> AMADLEQKVLEMEASTYDGVFIWKISDFPRKRQEAVAGRIPAIFSPAFYTSRYGYKMCLRIYLNGDGTGRGTHLSLFFVVMKGPNDALLRWPFNQKVTLMLLDQNNREHVIDAFRPDVT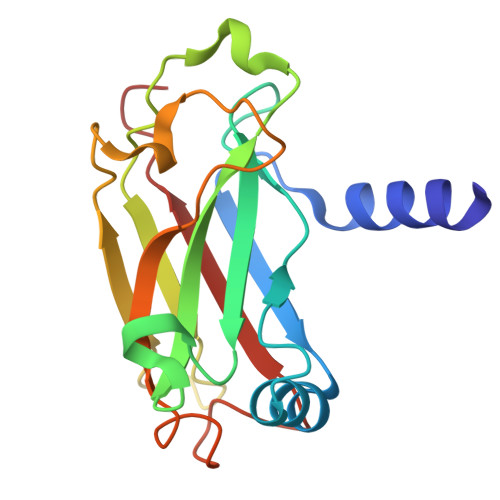SSSFQRPVNDMNIASGCPLFCPVSKMEAKNSYVRDDAIFIKAIVDLTGL> MLFTFFD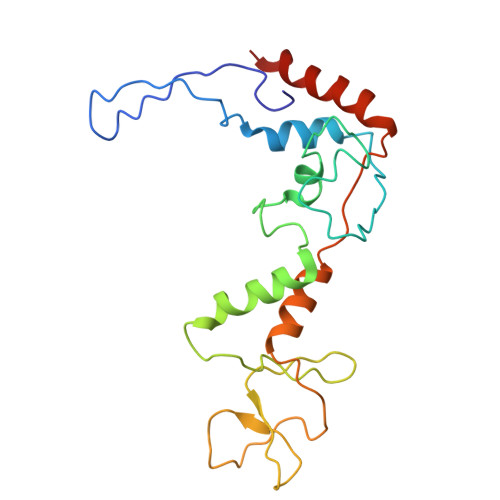PIEYAAKTVNKNAPTIPMTDIFRNYKDYFKRALAGYRLRTYYIKGSPRPEELANAIYGNPQLYWVLLMCNDNYDPYYGWITSQEAAYQASIQKYKNVGGDQIVYHVNENGEKFYNLISYDDNPYVWYDKGDKARKYPQYEGALAAVDTYEAAVLENEKLRQIKIIAKSDINSFMNDLIRIMEKSYGNDK> GEELYEV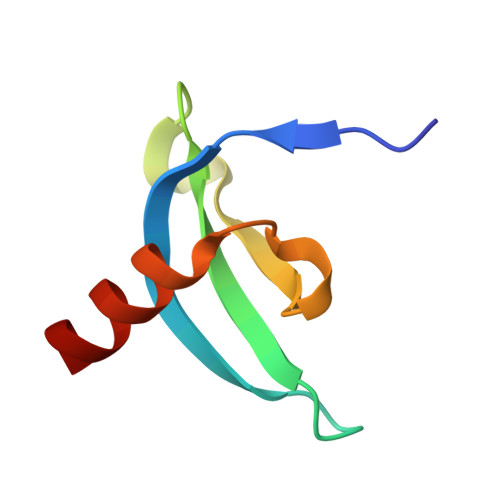ERIVDKRKNKKGKTEYLVRWKGYDSEDDTWEPEQHLVNCEEYIHDFNRRH>[4x]MVTARLRPELAGLPVYVPGKTVPGAIKLAS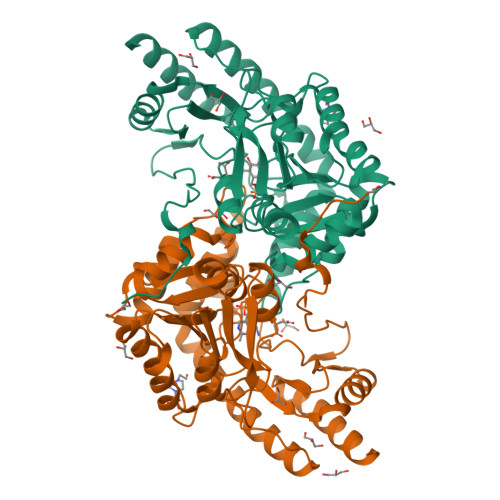NETVFGPLPSVRAAIDRATDTVNRYPDNGCVQLKAALARHLGPDFAPEHVAVGCGSVSLCQQLVQVTASVGDEVVFGWRSFELYPPQVRVAGAIPIQVPLTDHTFDLYAMLATVTDRTRLIFVCNPNNPTSTVVGPDALARFVEAVPAHILIAIDEAYVEYIRDGMRPDSLGLVRAHNNVVVLRTFSKAYGLAGLRIGYAIGHPDVITALDKVYVPFTVSSIGQAAAIASLDAADELLARTDTVVAERARVSAELRAAGFTLPPSQANFVWLPLGSRTQDFVEQAADARIVVRPYGTDGVRVTVAAPEENDAFLRFARRWRSDQKLAAALEHHHHHH4-[2-(4-methylpentyl)-1,3-thiazol-4-yl]-~{N}-[3,3,3-tris(fluoranyl)propyl]benzamide 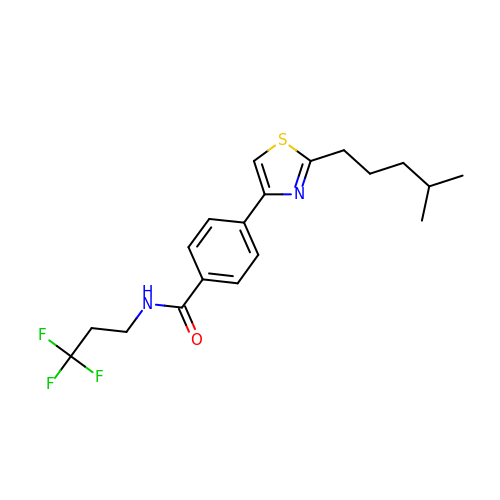| C19 H23 F3 N2 O S | KTLILWGHLTVHAZ-UHFFFAOYSA-N>MIVIFVDFDYFFAQVEEVLNPQYKGKPLVVCVYSGRTKTSGAVATANYEARKLGVKAGMPIIKAMQIAPSAIYVPMRKPIYEAFSNRIMNLLNKHADKIEVASIDEAYLDVTNKVEGNFENGIELARKIKQEILEKEKITVTVGVAPNKILAKIIADKSKPNGLGVIRPTEVQDFLNELDIDEIPGIGSVLARRLNELGIQKLRDILSKNYNELEKITGKAKALYLLKLAQDEYNEPIRTRVRKSIGRYLTLPYNTRDVKVILPYLKKAINEAYNKVNGIPMRITVIAIMEDLDILSKGKKFKHGISIDNAYKVAEDLLRELLVRDKRRN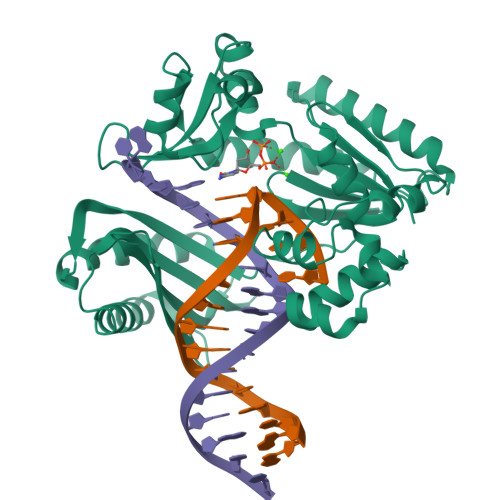VRRIGVKLDNIIINKTNLSDFFDIGGHHHHHH[2x]(2S,5R)-5-amino-1-formyl-5-hydroxy-N-(piperidin-4-yl)piperidine-2-carboxamide | C12 H22 N4 O3 | 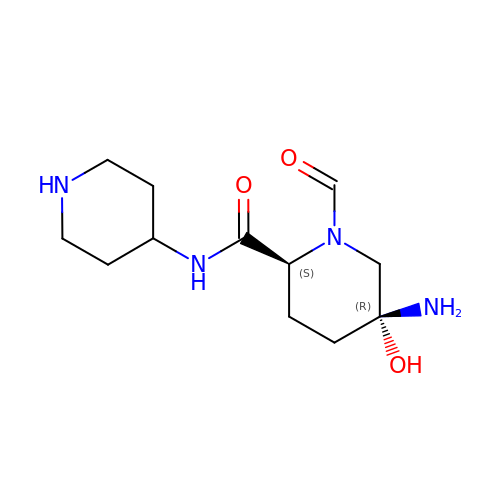SWVCDWJYHKCKJJ-CMPLNLGQSA-N2-(2-oxopyrrolidin-1-yl)-N-(1,3-thiazol-2-yl)acetamide | C9 H11 N3 O2 S | 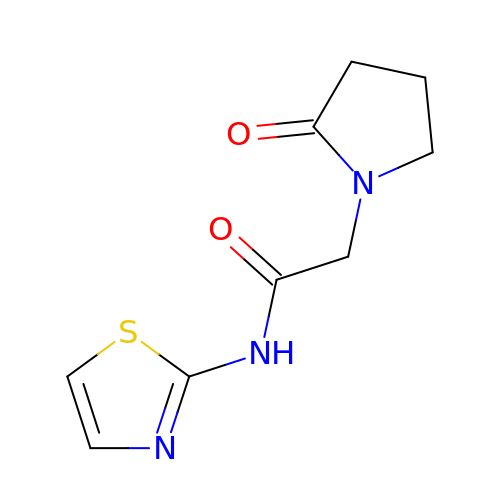JHZYBLIEJWESOZ-UHFFFAOYSA-N> MSARISLFAVVVEDMAKSMEFYRKMGVEIPAEADSAPHTEAVLDGGIRLAWDT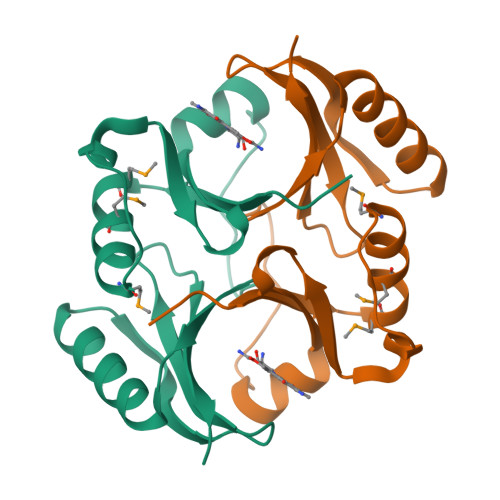VETVRSYDPEWQAPTGGHRFAIAFEFPDTASVDKKYAELVDAGYEGHLKPWNAVWGQRYAIVKDPDGNVVDLFAPLP> LVHVASVEKGRSYEDFQKVYNAIALKLREDDEYDNYIGYGPVLVRLAWHTSGTWDKHDNTGGSYGGTYRFKKEFNDPSNAGLQNGFKFLEPIHKEFPWISSGDLFSLGGVTAVQEMQGPKIPWRCGRVDTPEDTTPDNGRLPDADKDADYVRTFFQRLNMNDREVVALMGAHALGKTHLKRSGY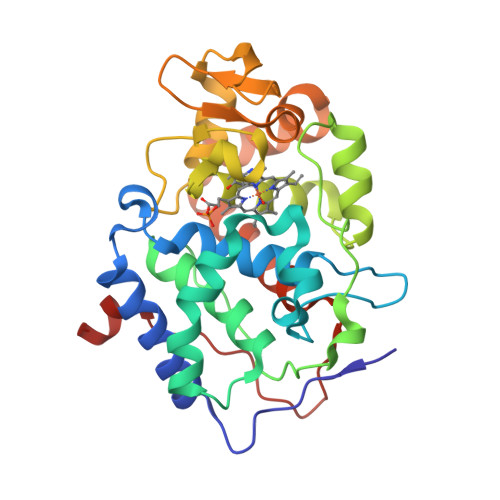EGPWGAANNVFTNEFYLNLLNEDWKLEKNDANNEQWDSKSGYMMLPTDYSLIQDPKYLSIVKEYANDQDKFFKDFSKAFEKLLENGITFPKDAPSPFIFKTLEEQGL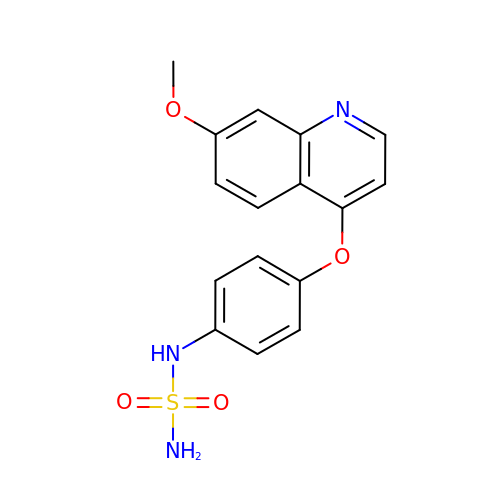N-{4-[(7-methoxyquinolin-4-yl)oxy]phenyl}sulfuric diamide | C16 H15 N3 O4 S | YDPVHBWULHMYJX-UHFFFAOYSA-N Uniquely among microbes to date, P. gingivalis also produces a secreted PAD (called PPAD18), which protects P. gingivalis during acidic cleansing in the mouth through ammonia generated during host and endogenous protein citrullination. PPAD does not require calcium for catalysis and is genetically unrelated with animal PADs and, like the latter and cysteine peptidases, its main catalytic residue is a cysteine (C351 in PPAD20). In contrast, PPAD citrullinates C-terminal arginines like those generated by the prior action of Rgps17, which may be facilitated by the surface co-localization of Rgps and PPAD20.

We further obtained a substrate-mimic complex of DTDP-untreated wt PPAD with dipeptide aspartate-glutamine, and a true substrate complex of DTDP-untreated PPAD–C351A with dipeptide methionine-arginine. The complex structures are equivalent, including the backbone of the bound dipeptides, except for some minimal displacement and the differing side chains, so the substrate complex is taken hereafter as reference except for issues dealing with C351Sγ, for which the substrate-mimic complex will be referred to. Comparison with the substrate-free structure revealed overall coincidence of the complexes except for the rearrangement of the Michaelis loop (maximal displacement 7.5 Å at N230Cα), which adopts a closed conformation that traps the substrate arginine side chain. This causes H196 to be rotated ~100° around its χ1 angle toward bulk solvent and Y233 to be displaced by 4.1 Å and slightly reoriented for its side chain to bind the substrate (see below). The guanidinium group is further tightly bound by D238 through a double salt bridge with arginine Nη1 and Nη2 atoms (2.9 Å and 3.0 Å), by the main-chain carbonyl of T346 (3.2 Å away from atom Nη1), and by D130 through a second double salt bridge with arginine Nε and Nη2 atoms (2.8 Å and 2.9 Å). The aliphatic part of the arginine is bound between the hydrophobic side chains of I234 and W127 (both 3.7 Å apart). The C-terminal carboxylate is linked by a double salt bridge with R152Nη2 (3.0 Å) and Nε (2.8 Å). In addition, one of the carboxylate oxygens is further bound by R154Nη1 (2.9 Å) and the other by Y233Oη (2.8 Å). In addition, these interactions draw an intricate network to fix the substrate in the cleft, which makes it difficult to imagine how a substrate with C-terminal extension to the arginine, i.e. an endodeiminase substrate, would be bound by PPAD, as a C-terminally extended peptide would collide with Y233 and R152 side chains.

> AFQETNPPAGPVRAIAEYERSAAVLVRYPFGIPMELIKELAKNDKVITIVASESQKNTVITQYTQSGVNLSNCDFIIAKTDSYWTRDYTGWFAMYDTNKVGLVDFIYNRPRPNDDEFPKYEAQYLGIEMFGMKLKQTGGNYMTDGYGSAVQSHIAYTENSSLSQAQVNQKMKDYLGITHHDVVQDPNGEYINHVDCWGKYLAPNKILIRKVPDNHPQHQALEDMAAYFAAQTCAWGTKYEVYRALATNEQPYTNSLILNNRVFVPVNGPASVDNDALNVYKTAMPGYEIIGVKGASGTPWLGTDALHARTHEVADKGYLYIKHYPILGEQAGPDYKIEADVVSCANATISPVQCYYRINGSGSFKAADMTMESTGHYTYSFTGLNKNDKVEYYISAADNSGRKETYPFIGEPDPFKFTCMNETNTCTVTGAA> MRILVCAKQVPDTNEVKIDPKTG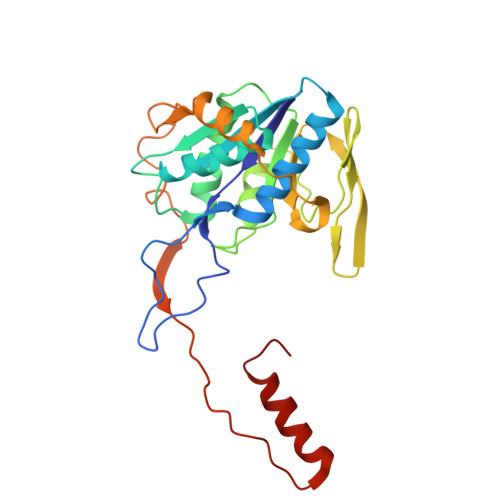TMIREGVPSILNPDDANALEAALVIKDENPGTEVIVMTMGPPQASEMLRECLAMGADEAYLLSDRAFGGADTWATSATLAAGIKKVKKVDLVLAGRQAIDGDTAQVGSQIAQRLKMPVVTYVEDIKIEDKKAIVHRQMEDGYEVIEVQLPCLLTCVKELNDPRYMSVGGIMDAYEQPITIWNHEDIGLSPEACGLNASPTQVFRSFSPPAKGGGEMITGTTVNEVAGSLVSKLKEKHII> ETSYTLNEVVPL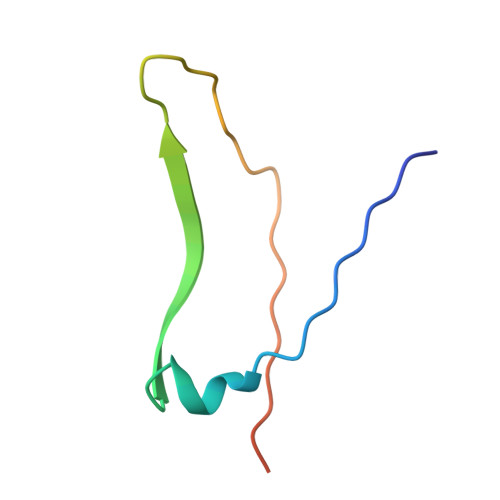KEFVPEWVRIGFSATTGAEFAAHEVLSWYFHSELAGTSSS3-(beta-D-glucopyranosyl)-6-propylfuro[2,3-d]pyrimidin-2(3H)-one | C15 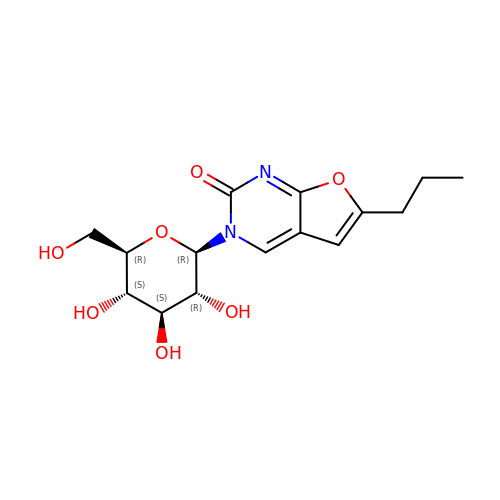H20 N2 O7 | XKVQKUGUMPARLW-YGEZULPYSA-N URIDINE-DIPHOSPHATE-2(N-ACETYLGLUCOSAMINYL-3-FLUORO-2-PHOSPHONOOXY)PROPIONIC ACID | C20 H31 F N3 O23 P3 | 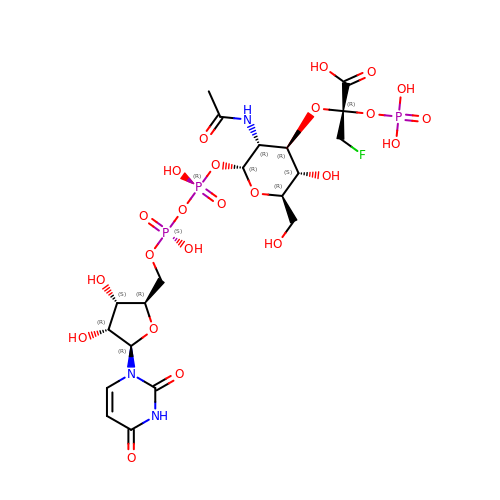FUDVRUWZNPQAFR-BVDGEXFOSA-N> MSLPLLRPFETVSLENAVEDLVVRFILNVPPEDLSTVERVLFHFEEASWFYTDFVKLMNPYLPNLSIKSFSKIVIDICPLIWNWDITPENALVKFSNYKKTIPVRGAAIFNDSLSKILLLRGINSKHWSFPRGKIGKDEDDVACCIREVKEETGFDLTGFIDADQYVERNMNGKNFKIFLVKGVPEDFEFKPEHKNEIQAIEWKDFKKLSKAITKNEGSAKVFLVNSMIRPLSLYVKNEKRAKDENKLK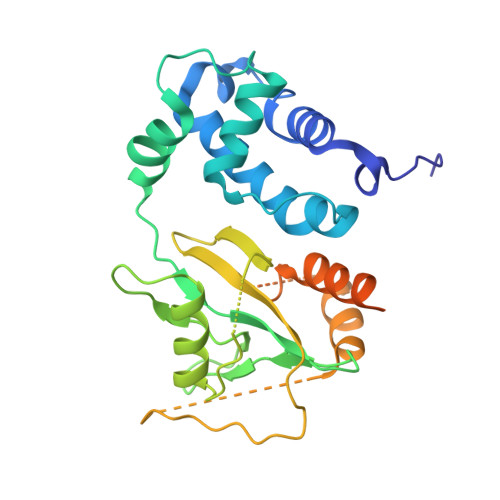LYAEEHLKSILGLNKKENKIVLDAGRHHHHHH> MSLNYKNYTVMLVDDEQPILNSLKRLIKRLGCNIITFTSPLD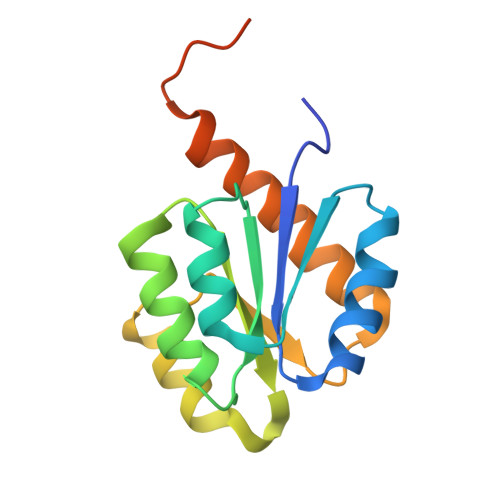ALEALKGTSVQLVISDMRMPEMGGEVFLEQVAKSYPDIERVVISGYADAQATIDAVNRGKISRFLLKPWEDEDVFKVVEKGLQLAFLREENLRLQEETEAKNKQEGHHHHHH>[6x]MSRSSATLIGFTAILLWSTLALATSSTGAVPPFLLTALTFTIGGAVGIAAGLARGVGLSVLRQPWPVWVHGIGGLFGYHFFYFSALKLAPPAEAGLVAYLWPLLIVLFSAFLPGERLRPAHVAGALMGLAGTVVLLGARAGGFG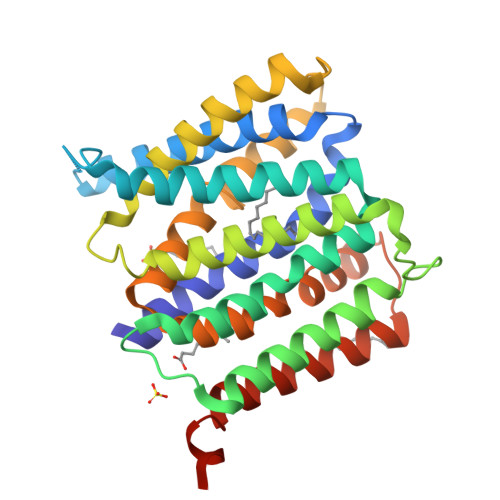FAPEYVPGYLAAAACAVIWSVYSVASRRFARVPTEVVAGFCLATAALSALCHILFEPSVWPVGSEWLAVVALGIGPVGIAFYTWDIGMKRGDVRLLGVLSYAAPVLSTLLLVVAGFAAPSGALAIACALIVGGAAVATLLARRLESSGENLYFQ> AETVESCLAKSHTE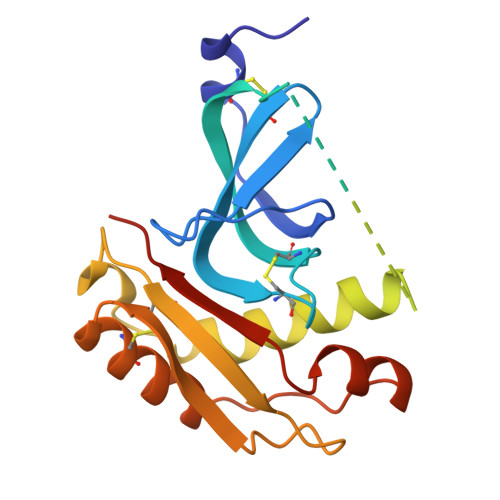NSFTNVWKDDKTLDRYANYEGCLWNATGVVVCTGDETQCYGTWVPIGLAIPENEGGGSEGGGSEGGGSEGGGDDIFGELSSGKNAPKTGGGAKGNNASPAGSGNTKNNGASGADINNYAGQIKSAIESKFYDASSYAGKTCTLRIKLAPDGMLLDIKPEGGDPALCQAALAAAKLAKIPKPPSQAVYEVFKNAPLDFKPAAAHHHHHH> MTVKVCVCGGGNGAHTLSGLAASRDGVEVRVLTLFADEAERWTKALGADELTVIVNEKDGTQTEVKSRPKVITKDPEIAISGADVVILTVPAFAHEGYFQAMAPYVQDSALIVGLPSQAGFEFQCRDILGDKAAAVSMMSFETLPWACRIKEFGRKVEVLGTKSVLAASLIKGTAKTVDPLSTLQMLHGAEPVFRLAKHFLEMLIMSYSFVHPAILFGRWGSWDGKPVPEAPLFYQGIDQATADMLTACSNECKDVANAIMAACPGNDLSDVKDIYQWYLEYYHEDIQDDHDLYHAITTNKSYKGLVHPVKAVDGGVAPDFGNRYLTEDIPMGMIVFKGVA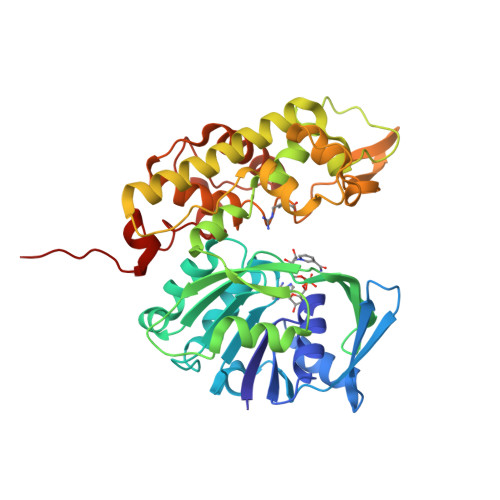IAAGVAIPSNDKLIMWAQEKIGKEYLVDGALTGKDVATTRCPQRYGFNTLDAILTGKKHHHHH>IGMAPGGYVAPKAVWLPAVKAKGLEISGTFTHRQGHIYMEMNFTNKALQHMTDFAIQFNKNSFGVIPSTPLAIHTPLMPNQSIDVSLPLNTLGPVMKMEPLNNLQVAVKNNIDVFYFSCLIPLNVLFVEDGKMERQVFLATWKDIPNENELQFQIKECHLNADTVSSKLQNNNVYTIAKRNVEGQDMLYQSL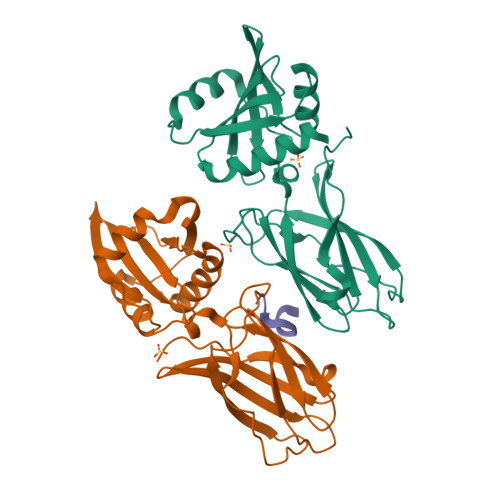KLTNGIWILAELRIQPGNPNYTLSLKCRAPEVSQYIYQVYDSILKN[2x];> SFGDGFADFSTL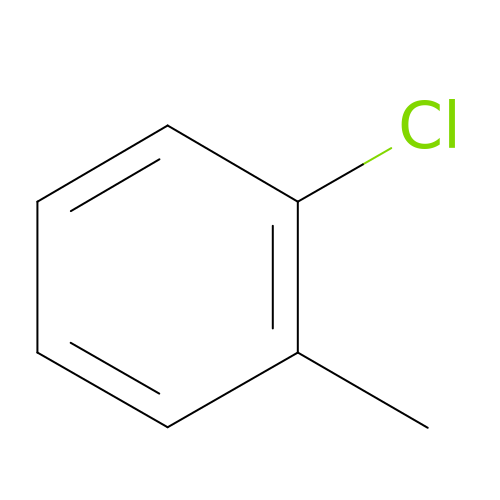1-chloranyl-2-methyl-benzene | C7 H7 Cl | IBSQPLPBRSHTTG-UHFFFAOYSA-N>SHMPDQRQTRFAHITKAHPCFNEKLHDRVGRVHVPIAPRCNIHCKFCTRDINECERRPGVTGRLMTADDAIKHVEKVKEEMPISVIGVAGPGDALANEETFEFFKKASKKFPDLLKCMSTNGLLLPDRADELAELGINTVTVTVNAVDPEIGEKIYSFVVYKDKVYHGREAFEVLSRNQLEGIEKLAERGIIVKVNSVLIPGLNDEHIVDIAREVKKRGASLMNI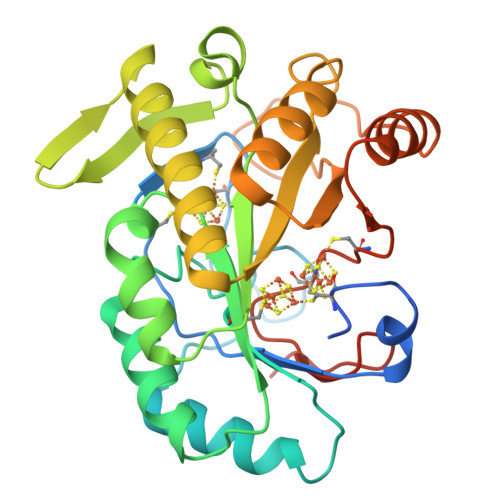IPLIPMGEMKDYPRPTCEQIERVRNEVEKIIPVFRACTQCRADAYGIPGKKEADKHLDMTPASHY[2x]> MWIIEAEGDILKGKSRILFPGTYIVGRNVSDDSSHIQVISKSISKRHARFTILTPSEKDYFTGGPCEFEVKDLDTKFGTKVNEKVVGQNGDSYKEKDLKIQLGKCPFTINAYWRSMCIQFDNPEMLSQWASNLNLLGIPTGLRDSDATTHFVMNRQAGSSITVGTMYAFLKKTVIIDDSYLQYLSTVKESVIEDASLMPDALECFKNIIKNNDQFPSSPEDCIN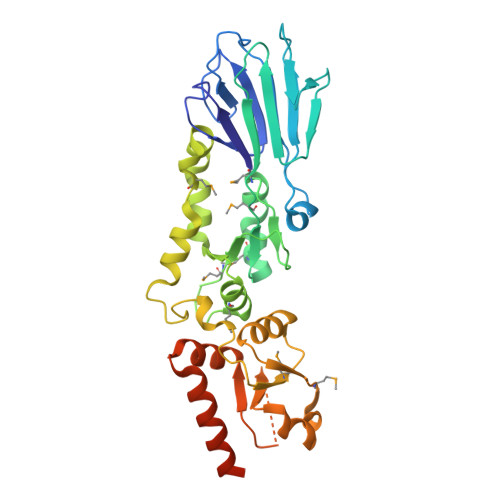SLEGFSCAMLNTSSESHHLLELLGLRISTFMSLGDIDKELISKTDFVVLNNAVYDSEKISFPEGIFCLTIEQLWKIIIERNSRELISKEIERLKYATASNSTPQKIAAALEHHHHHH> ALMDGTAAEPRPGAGSLQHAQPPPQPRKKRPEDFKFGKILGEGSFSTVVLARELATSREYAIKILEKRHIIKENKVPYVTRERDVMSRLDHPFFVKLYFTFQDDEKLYFGLSYAKNGELLKYIRKIGSFDETCTRFYTAEIVSALEYLHGKGIIHRDLKPENILLNEDMHIQITDFGTAKVLSPESKQARANSFVGTAQYVSPELLTEKSACKSSDLWALGCII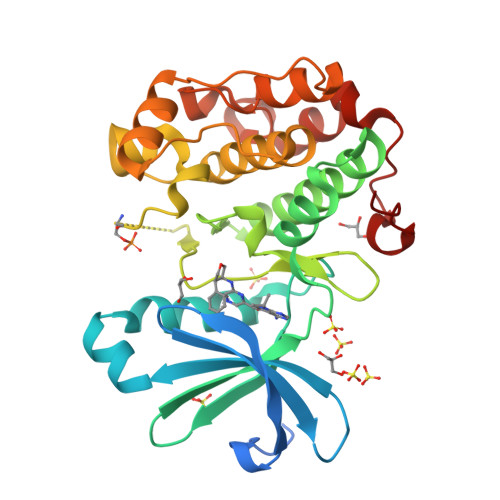YQLVAGLPPFRAGNEYLIFQKIIKLEYDFPEKFFPKARDLVEKLLVLDATKRLGCEEMEGYGPLKAHPFFESVTWENLHQQTPPKLT> MFNKSFGTPFGGGTGGFGTTSTFGQNTGFGTTSGGAFGTSAFGSSNNTGGLFGNSQTKPGGLFGTSSFSQPATSTSTGFGFGTSTGTANTLFGTASTGTSLFSSQNNAFAQNKPTGFGNFGTSTSSGGLFGTTNTTSNPFGSTSGSLFGPSSFTAAPTGTTIKFNPPTGTDTMVKAGVSTNISTKHQCITAMKEYESKSLEELRLEDYQANRKGPQNQVGAGTTTGLFGSSPATSSATGLFSSSTTNSGFAYGQNKTAFGTSTTGFGTNPGGLFGQQNQQTTSLFSKPFGQATTTQNTGFSFGNTSTIGQPSTNTMGLFGVTQASQPGGLFGTATNTSTGTAFGTGTGLFGQTNTGFGAVGSTLFGNNKLTTFGSSTTSAPSFGTTSGGLFGNKPTLTLGTNTNTSNFGFGTNTSGNSIFGSKPAPGTLGTGLGAGFGTALGAGQASLFGNNQPKIGGPLGTGAFGAPGFNTTTATLGFGAPQAPVALTDPNASAAQQAVLQQHINSLTYSPFGDSPLFRNPMSDPKKKEERLKPTNPAAQKALTTPTHYKLTPRPATRVRPKALQTTGTAKSHLFDGLDDDEPSLANGAFMPKKSIKKLVLKNLNNSNLFSPVNRDSENLASPSEYPENGERFSFLSKPVDENHQQDGDEDSLVSHFYTNPIAKPIPQTPESAGNKHSNSNSVDDTIVALNMRAALRNGLEGSSEETSFHDESLQDDREEIENNSYHMHPAGIILTKVGYYTIPSMDDLAKITNEKGECIVSDFTIGRKGYGSIYFEGDVNLTNLNLDDIVHIRRKEVVVYLDDNQKPPVGEGLNRKAEVTLDGVWPTDKTSRCLIKSPDRLADINYEGRLEAVSRKQGAQFKEYRPETGSWVFKVSHFSKYGLQDSDEEEEEHPSKTSTKKLKTAPLPPASQTTPLQMALNGKPAPPPQSQSPEVEQLGRVVELDSDMVDITQEPVLDTMLEESMPEDQEPVSASTHIASSLGINPHVLQIMKASLLTDEEDVDMALDQRFSRLPSKADTSQEICSPRLPISASHSSKTRSLVGGLLQSKFTSGAFLSPSVSVQECRTPRAASLMNIPSTSSWSVPPPLTSVFTMPSPAPEVPLKTVGTRRQLGLVPREKSVTYGKGKLLMDMALFMGRSFRVGWGPNWTLANSGEQLNGSHELENHQIADSMEFGFLPNPVAVKPLTESPFKVHLEKLSLRQRKPDEDMKLYQTPLELKLKHSTVHVDELCPLIVPNLGVAVIHDYADWVKEASGDLPEAQIVKHWSLTWTLCEALWGHLKELDSQLNEPREYIQILERRRAFSRWLSCTATPQIEEEVSLTQKNSPVEAVFSYLTGKRISEACSLAQQSGDHRLALLLSQFVGSQSVRELLTMQLVDWHQLQADSFIQDERLRIFALLAGKPVWQLSEKKQINVCSQLDWKRSLAIHLWYLLPPTASISRALSMYEEAFQNTSDSDRYACSPLPSYLEGSGCVIAEEQNSQTPLRDVCFHLLKLYSDRHYDLNQLLEPRSITADPLDYRLSWHLWEVLRALNYTHLSAQCEGVLQASYAGQLESEGLWEWAIFVLLHIDNSGIREKAVRELLTRHCQLLETPESWAKETFLTQKLRVPAKWIHEAKAVRAHMESDKHLEALCLFKAEHWNRCHKLIIRHLASDAIINENYDYLKGFLEDLAPPERSSLIQD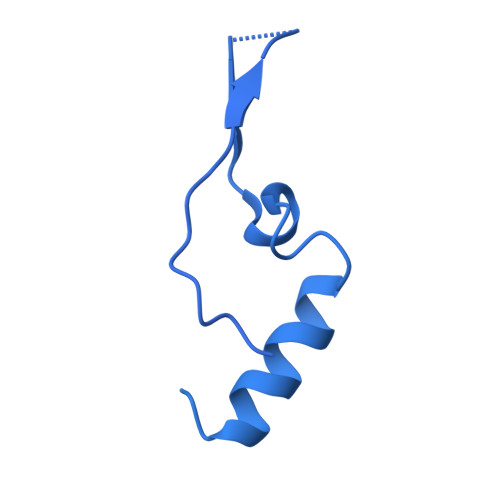WETSGLVYLDYIRVIEMLRHIQQVDCSGNDLEQLHIKVTSLCSRIEQIQCYSAKDRLAQSDMAKRVANLLRVVLSLHHPPDRTSDSTPDPQRVPLRLLAPHIGRLPMPEDYAMDELRSLTQSYLRELAVGSL>SMKDENKLNVRMLSDVCMQSRLLKEALESKLPLALEITPFSELWLEENKPESRSIQMLVIDYSRISDDVLTDYSSFKHISCPDAKEVIINCPQDIEHKLLFKWNNLAGVFYIDDDMDTLIKGMSKILQDEMWLTRKLAQEYILHYRAGNSVVTSQMYAKLTK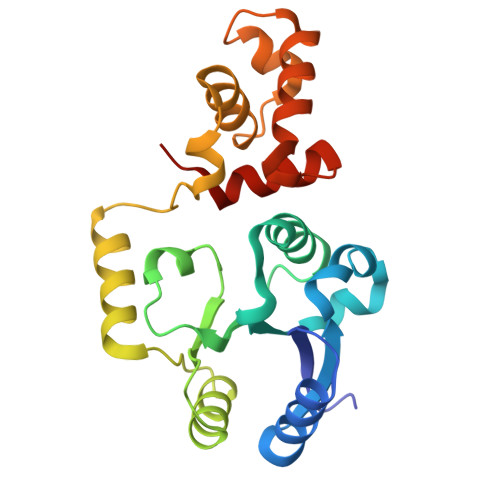REQQIIKLLGSGASNIEIADKLFVSENTVKTHLHNVFKKINAKNRLQALIWAKNNIGIEEVNS[4x]>[2x]SNAMSIEKVPILGKETIHVGYGIADHIVREVIANLASSTYVIVTDTNMARTPQYSKLTDDFKTNLSEKRPESRLLTYCVSPGENNKNRATKAAVEDFLLQQGCTRDTVILAVGGGVIGDMIGFVAATFMRGVRVVQVPTTLLAMVDSSVGGKTAIDTPLGKNFIGAFHQPEYVFCDVSFLETLPARQFINGMAEVVKTAAIWNEEEFTRLENFSKKFLSVVTSKKPDLQSIKAELVKTVLESVRVKAGVVSSDEKEAGLRNLLNFGHTIGHAIEAVLTPEALHGECVSIGMIKEAELSRYLGILPPVAVARLSKCLVAYGLPVSIDDKEFLKKVGPKRHYVEIDILLKKMAIDKKNDGSKIRCVLLEKIGKCYQLKAHQVSKQDLSFVLT

In the human fungal pathogen Candida albicans, ARO1 encodes an essential multi-enzyme that catalyses consecutive steps in the shikimate pathway for biosynthesis of chorismate, a precursor to folate and the aromatic amino acids. In Fungi and Apicomplexa, the second to the sixth steps of the shikimate pathway are supported by five enzymatic domains combined in a single protein known as Aro1 or AroM. Aro1 forms a flexible dimer allowing relative autonomy of enzymatic function of the individual domains. Our activity and in cellulo data suggest that only four of Aro1’s enzymatic domains are functional and essential for viability of C. albicans, whereas the 3-dehydroquinate dehydratase (DHQase) domain is inactive because of active site substitutions.

Aro1DHQS was crystallised in the presence of its cofactor NADH. Accordingly, in addition to the two copies of this domain found in the asymmetric unit we identified unambiguous additional electron density corresponding to one NADH molecule bound to each copy of this fragment. Notably, the residues that interact with the 3-dehydroquinate analog carbaphosphonate, NADH, and Zn2+ as observed in the A. nidulans AroMDHQS structure are completely conserved in the Aro1DHQS active site. Specifically, Aro1DHQS residues H264, H268, and H280 coordinate the catalytic Zn2+, allowing for identification of potential catalytic residues of Aro1. The two Aro1DHQS chains in the asymmetric unit formed a dimer with over 1,100 Å2 buried surface area. The two corresponding domains in the fungal AroM multi-enzymes showed very similar dimeric arrangements, along with the single-domain DHQS enzymes listed above. The interface between the Aro1DHQS domains in the Aro1 dimer is the same as seen in the Aro1DHQS crystal structure.>GSMENTDVFLGLHDFLERMRKPSAGDFVKSIKSFIVSFSNNAPDPEKDCAMVQEFFSKMEAAFRAHPLWSGCSEEELDSAGDGLEKYVMTKLFTRVFASNTEEVIADEKLFQKMSLVQQFISPENLDIQPTFQNESSWLLAQKELQKINMYKAPRDKLVCILNCCKVINNLLLNASIASNENAPGADEFLPVLIYVTIKANPPQLHSNLLYIQRYRRESKLVGEAAYFFTNILSAESFISNIDAKSISLDEAEFEKNMESARARISG[2x];>[2x]GSMAAAGNKSINAKLVLLGDVGAGKSSLVLRFVKDQFVEFQESTIGAAFFSQTLAVNDATVKFEIWDTAGQERYHSLAPMYYRGAAAAIIVFDVTN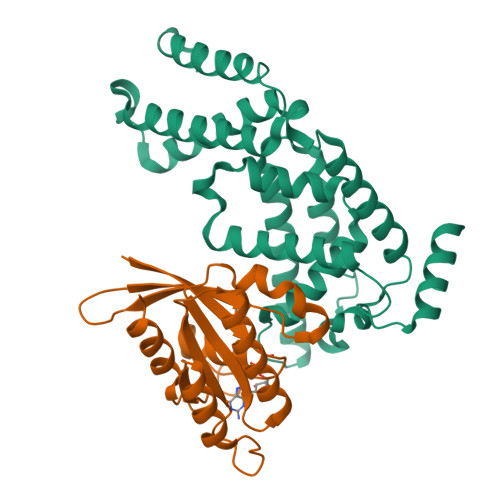QASFERAKKWVQELQAQGNPNMVMALAGNKSDLLDARKVTAEDAQTYAQENGLFFMETSAKTATNVKEIFYEIARRLPRVQPTEN> GFPCGESCVYGPCFTAAIGCSCKSKVCYKN;> GFPC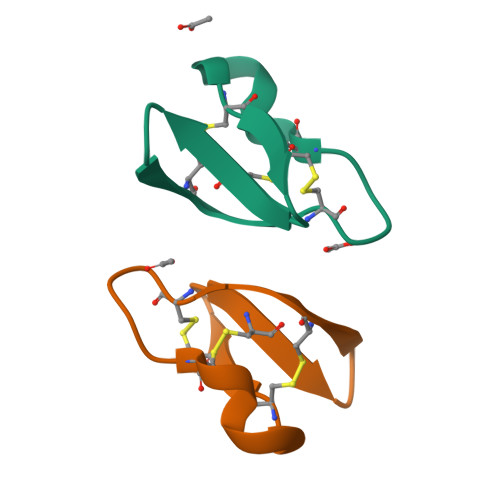GESCVYLPCFTAAIGCSCKSKVCYKN>EPVKFKDCGSWVGVIKEVNVSPCPTQPCKLHRGQS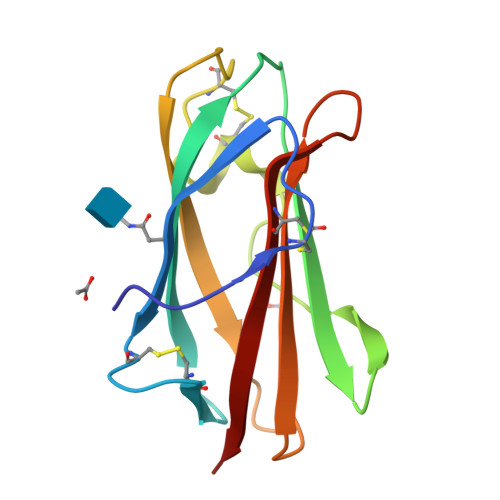YSVNVTFTSNTQSQSSKAVVHGIVMGIPVPFPIPESDGCKSGIRCPIEKDKTYNYVNKLPVKNEYPSIKVVVEWELTDDKNQRFFCWQIPIEVEA[3x]> MPRVVPDQRSKFENEEFFRKLSRECEIKYTGFRDRPHEERQTRFQNACRDGRSEIAFVATGTNLSLQFFPASWQGEQRQTPSREYVDLEREAGKVYLKAPMILNGVCVIWKGWIDLHRLDGMG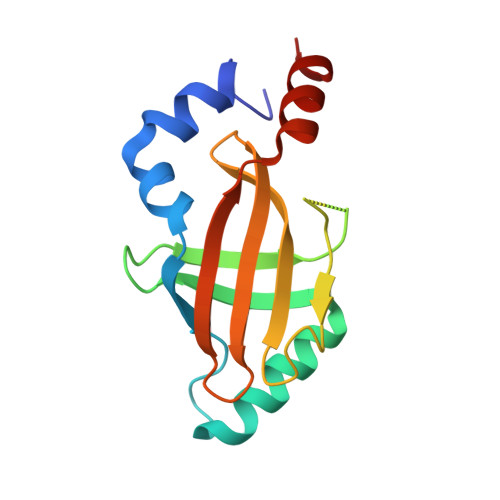CLEFDEERAQQEDALAQQ> HHHHHHGDAPGGAHMTAQTVTGAVAAAQLGATLPHEHVIFGYPGYAGDVTLGPFDHAAALASCTETARALLARGI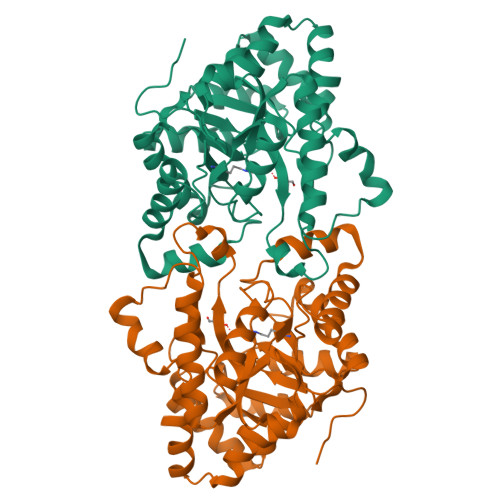QTVVDATPNDCGRNPAFLREVSEATGLQILCATGFWYEGEGATTYFKFRASLGDAESEIYEMMRTEVTEGIAGTGIRAGVIKLASSRDAITPYEQLFFRAAARVQRETGVPIITHTQEGQQGPQQAELLTSLGADPARIMIGHMDGNTDPAYHRETLRHGVSIAFDRIGLQGMVGTPTDAERLSVLTTLLGEGYADRLLLSHDSIWHWLGRPPAIPEAALPAVKDWHPLHISDDILPDLRRRGITEEQVGQMTVGNPARLFG(S)-4-ISOPROPOXYCARBONYL-6-METHOXY-3-METHYLTHIOMETHYL-3,4-DIHYDROQUINOXALIN-2(1H)-THIONE | C15 H20 N2 O3 S2 | 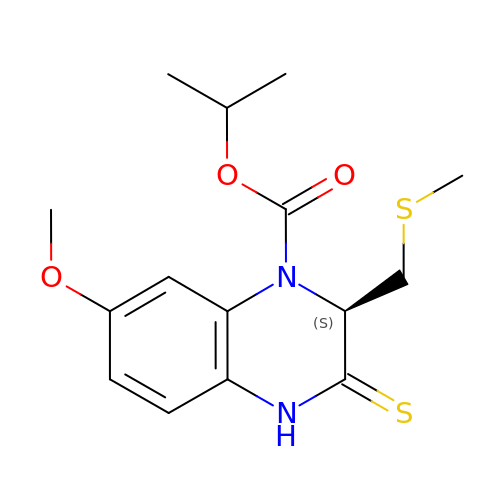GWKIPRVERALPRD-ZDUSSCGKSA-N> MTEETISQAVPPVRDWPAVDLPGSDFDPVLTELMREGPVTRISLPNGEGWAWLVTRHDDVRLVTNDPRFGREAVMDRQVTRLAPHFIPARGAVGFLDPPDHTRLRRSVAAAFTARGVERVRERSRGMLDELVDAMLRAGPPADLTEAVLSPFPIAVI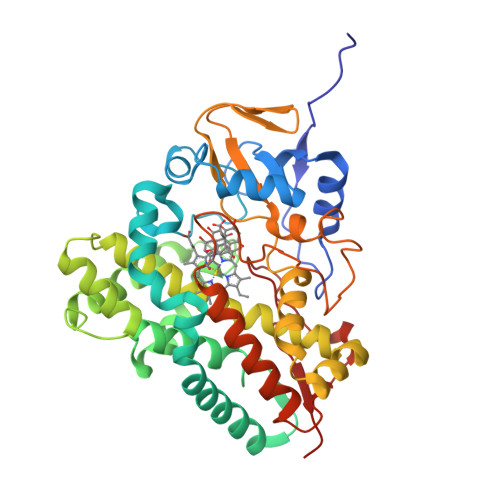CELMGVPATDRHSMHTWTQLILSSSHGAEVSERAKNEMNAYFSDLIGLRSDSAGEDVTSLLGAAVGRDEITLSEAVGLAVLLQIGGEAVTNNSGQMFHLLLSRPELAERLRSEPEIRPRAIDELLRWIPHRNAVGLSRIALEDVEIKGVRIRAGDAVYVSYLAANRDPEVFPDPDRIDFERSPNPHVSFGFGPHYCPGGMLARLESELLVDAVLDRVPGLKLAVAPEDVPFKKGALIRGPEALPVTWAA>MGSAIQDYFVKNRVGHSKPWESGKFKAADNFPDLSKHNNVMASQLTKELYEKYWDKVTPNGVTFDKCIQTGVDNPGNKFYGKKTGCVFGDEYSYECYKEFFDKCIEEIHHFKPSDKHPAPDLDHNKLVGGVFEDKYVKSCRIRCGRSVKGVCLPPAMSRAERRLVEKVVSDALGGLKGDLAGKYYPLTTMNEKDQEQLIEDHFLFEKPTGALLTTSGCARDWPDGRGIWHNNEKNFLVWINEEDHIRVISMQKGGDLKAVFSRFARGLLEVERLMKECGHGLMHNDRLGYICTCPTNMGTVVRASVHLRLAFLEKHPRFDEMLGKLRLGK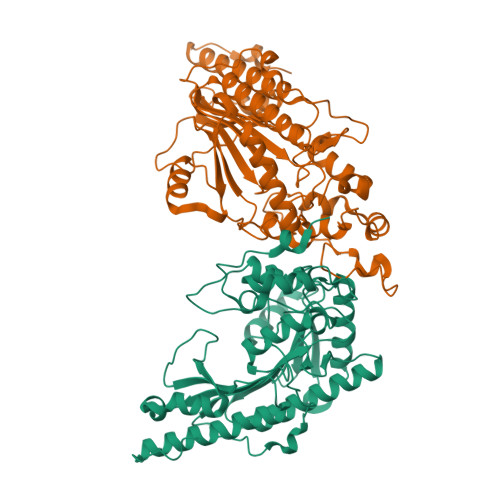RGTGGESSLATDSTYDISNWARLGKSERELVQVLVDGVNLLIACDKKLEAGQSIDDMIPK[4x]>[2x]DHQVKDSLEQLRCHFTWELSIDDDEMPDLENRVLDQIEFLDTKYSVGIHNLLAYVKHLKGQNEEALKSLKEAENLMQEEHDNQANVRSLVTWGNFAWMYYHMGRLAEAQTYLDKVENICKKLSNPFRYRMECPEIDCEEGWALLKCGGKNYERAKACFEKVLEVDPENPESSAGYAISAYRLDGFKLATKNHKPFSLLPLRQAVRLNPDNGYIKVLLALKLQDEGQEAEGEKYIEEALANMSSQTYVFRYAAKFYRRKGSVDKALELLKKALQETPTSVLLHHQIGLCYKAQMIQIKEATKGQPRGQNREKLDKMIRSAIFHFESAVEKKPTFEVAHLDLARMYIEAGNHRKAEENFQKLLCMKPVVEETMQDIHFHYGRFQEFQKKSDVNAIIHYLKAIKIEQASLTRDKSINSLKKLVLRKLRRKALDLESLSLLG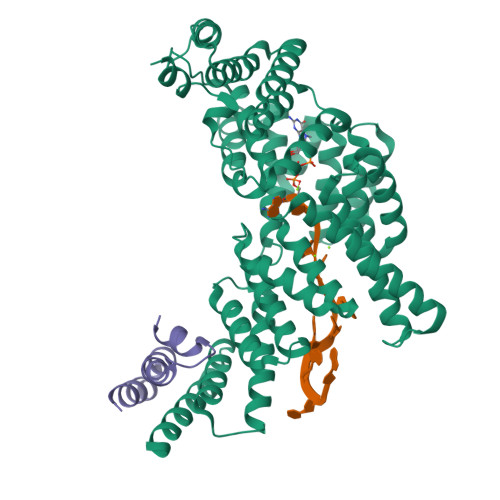FVYKLEGNMNEALEYYERALRLAADFE;>[2x]NYWYLQGLIHKQNGDLLQAAKCYEKELGRLLRDAPSGIGSIFLS>MVSKIRTFGWVQNPGKFENLKRVVQVFDRNSKVHNEVKNIKIPTLVKESKIQKELVAIMNQHDLIYTYKELVGTG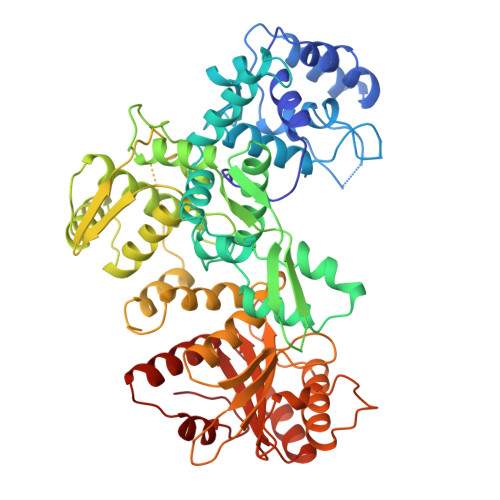TSIRSEAPCDAIIQATIADQGNKKGYIDNWSSDGFLRWAHALGFIEYINKSDSFVITDVGLAYSKSADGSAIEKEILIEAISSYPPAIRILTLLEDGQHLTKFDLGKNLGFSGESGFTSLPEGILLDTLANAMPKDKGEIRNNWEGSSDKYARMIGGWLDKLGLVKQGKKEFIIPTLGKPDNKEFISHAFKITGEGLKVLRRAKGSTKFTRVPKRVYWEMLATNLTDKEYVRTRRALILEILIKAGSLKIEQIQDNLKKLGFDEVIETIENDIKGLINTGIFIEIKGRFYQLKDHILQFVIPNRLGKPDLVKSELEEKKSELRHKLKYVPHEYIELIEIARNSTQDRILEMKVMEFFMKVYGYRGKHLGGSRKPDGAIYTVGSPIDYGVIVDTKAYSGGYNLPIGQADEMQRYVEENQTRNKHINPNEWWKVYPSSVTEFKFLFVSGHFKGNYKAQLTRLNHITNCNGAVLSVEELLIGGEMIKAGTLTLEEVRRKFNNGEINF[2x]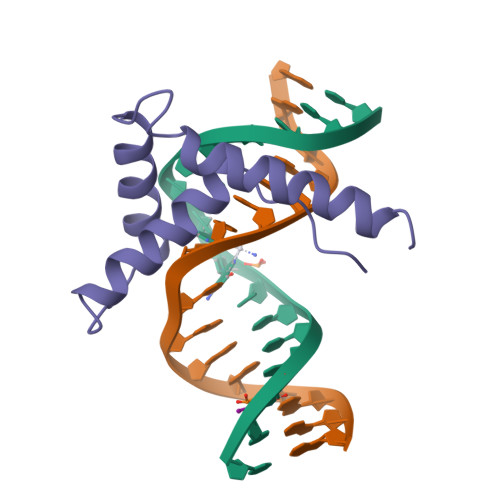> KPRGKMSSYAFFVQTCREEHKKKHPDASVNFSEFSKKCSERWKTMSAKEKGKFEDMAKADKARYEREMKTY> MNDDRETPPKRKPGEDDTLFDIDFLDDTTSHSGSRSKVTNSHANANYIPPSHVLPEETIDLDADDDNIENDVHENLFMSNNHDDQTSWNANRFDSDAYQPQSLRAVKPPGLFARFGNGLKNAFTFKRKKGPESFEMNHYNAVTNNELDDNYLDSRNKFNIKILFNRYILRKNVGDAEGNGEPRVIHINDSLANSSFGYSDNHISTTKYNFATFLPKFLFQEFSKYANLFFLCTSAIQQVPHVSPTNRYTTIGTLLVVLIVSAMKECIEDIKRANSDKELNNSTAEIFSEAHDDFVEKRWIDIRVGDIIRVKSEEPIPADTIILSSSEPEGLCYIETANLDGETNLKIKQSRVETAKFIDVKTLKNMNGKVVSEQPNSSLYTYEGTMTLNDRQIPLSPDQMILRGATLRNTAWIFGLVIFTGHETKLLRNATATPIKRTAVEKIINRQIIALFTVLIVLILISSIGNVIMSTADAKHLSYLYLEGTNKAGLFFKDFLTFWILFSNLVPISLFVTVELIKYYQAFMIGSDLDLYYEKTDTPTVVRTSSLVEELGQIEYIFSDKTGTLTRNIMEFKSCSIAGHCYIDKIPEDKTATVEDGIEVGYRKFDDLKKKLNDPSDEDSPIINDFLTLLATCHTVIPEFQSDGSIKYQAASPDEGALVQGGADLGYKFIIRKPNSVTVLLEETGEEKEYQLLNICEFNSTRKRMSAIFRFPDGSIKLFCKGADTVILERLDDEANQYVEATMRHLEDYASEGLRTLCLAMRDISEGEYEEWNSIYNEAATTLDNRAEKLDEAANLIEKNLILIGATAIEDKLQDGVPETIHTLQEAGIKIWVLTGDRQETAINIGMSCRLLSEDMNLLIINEETRDDTERNLLEKINALNEHQLSTHDMNTLALVIDGKSLGFALEPELEDYLLTVAKLCKAVICCRVSPLQKALVVKMVKRKSSSLLLAIGDGANDVSMIQAAHVGVGISGMEGMQAARSADIAVGQFKFLKKLLLVHGSWSYQRISVAILYSFYKNTALYMTQFWYVFANAFSGQSIMESWTMSFYNLFFTVWPPFVIGVFDQFVSSRLLERYPQLYKLGQKGQFFSVYIFWGWIINGFFHSAIVFIGTILIYRYGFALNMHGELADHWSWGVTVYTTSVIIVLGKAALVTNQWTKFTLIAIPGSLLFWLIFFPIYASIFPHANISREYYGVVKHTYGSGVFWLTLIVLPIFALVRDFLWKYYKRMYEPETYHVIQEMQKYNISDSRPHVQQFQNAIRKVRQVQRMKKQRGFAFSQAEEGGQEKIVRMYDTTQKRGKYGELQDASANPFNDNNGLGSNDFESAEPFIENPFADGNQNSNRFSSSRDDISFDI;> MVSLFKRGKAPPLTKEGPTSKKPPNTAFRQQRLKAWQPILSPQSVLPLLIFVACIFTPIGIGLIVSATKVQDLTIDYSHCDTKASTTAFEDIPKKYIKYHFKSKVENKPQWRLTENENGEQSCELQFEIPNDIKKSIFIYYKITNFYQNHRRYVQSFDTKQILGEPIKKDDLDTSCSPIRSREDKIIYPCGLIANSMFNDTFSQVLSGIDDTEDYNLTNKHISWSIDRHRFKTTKYNASDIVPPPNWMKKYPDGYTDENLPDIHTWEEFQVWMRTAAFPKFYKLTLKNESASLPKGKYQMNIELNYPISLFGGTKSFVLTTNGAIGGRNMSLGVLYLIVAGLCALFGIIFLVKLIFQPRAMGDHTYLNFDDEENEDYEDVHAENTTLREIL

The yeast lipid flippase Drs2p-Cdc50p is primarily found in the trans-Golgi network and is involved in protein trafficking between that network, the plasma membrane, and endosomes. Drs2p belongs to a large family of Type IV P-type ATPases (P4 ATPases). These enzymes translocate specific phospholipids from the extracellular side of the plasma membrane or from the lumenal side of internal organelles to the cytosolic side, creating and maintaining lipid compositional asymmetry in eukaryotic cell membranes. Drs2p-Cdc50p is activated by the binding of phosphatidylinositol 4-phosphate (PI4P), the Arf guanine nucleotide exchange factor Gea2p, and the Arf-related small-GTP-binding protein Arl1p to the C-terminal region of Drs2p9,10.

We obtained the activated complex by incubating the purified sample with 26 μM PI4P for 15 h at 4 °C, resulting in a cryo-EM structure determined at 3.3 Å resolution. We found that in vitro activation by PI4P was a very slow process; incubating the protein for a shorter period, say, 1-2 h, led to a mixture of activated and inactive conformations. Compared with the autoinhibited apo form, the active Drs2p-Cdc50p shows two major conformational changes: (1) the inhibitory C-tail of Drs2p is fully released from the extended horizontal groove in the regulatory A, N, and P domains of Drs2p and becomes disordered, and (2) the putative substrate-translocating path becomes more open, especially in the cytosolic side. In the structure of the active Drs2p-Cdc50p, the entire Drs2p C-tail becomes disordered, thus vacating the ATP-binding pocket of Drs2p previously occupied by Phe-1275 and Phe-1277. The A, N, and P domains in the activated conformation have all undergone rigid-body movement relative to the inhibited apo structure. Notably, the A domain, previously stabilized by the last stretch of the ordered inhibitory C-terminal peptide, has moved about 6 Å away from the P domain and has become partially flexible, as indicated by its weakened EM density. The A domain movement exposes the nucleotide-binding pocket in the N domain at the junction of the A, N, and P domains, perhaps priming the Drs2p structure for ATP entry, which is required for the lipid-flipping activity of the enzyme complex. Further, the rightward movement of the P domain has moved the cytosolic ends of TM3-6 by 1–2 Å, thereby resulting in a much more open substrate lipid-binding site in the cytosolic side. In the PI4P-activated structure, we found that this α-helix has swung 90°, away from the cytosolic regulatory A, N, and P domains on the left. Conceivably, such a swing motion will pull the inhibitory C-terminal peptide out of its horizontal groove and release it into solvent, hence releasing the inhibitory grip of the C-tail on the regulatory region.>APADNAADARPVDVSVSIFINKIYGVNTLEQTYKVDGYIVAQWTGKPRKTPGDKPLIVENTQIERWINNGLWVPALEFINVVGSPDTGNKRLMLFPDGRVIYNARFLGSFSNDMDFRLFPFDRQQFVLELEPFSYNNQQLRFSDIQVYTENIDNEEIDEWWIRGKASTHISDIRYDHLSSVQPNQNEFSRITVRIDAVRKIGYFVIQTYLPCIMTVILSQVSFWLNRESVPARTVFGVTTVLTMTTLSISARNSLPKVAYATAMDWFIAVCYAFVFSALIEFATVNYFTKRGVESVSKIDRLSRIAFPLLFGIFNLVYWATYLN[10x]

Type A γ-aminobutyric acid receptors (GABAARs) control neuronal excitability and are the primary inhibitory pentameric ligand-gated ion channels (pLGICs) in the central nervous system. GABAAR-mediated inhibition of neuronal excitability results from membrane hyperpolarization due to Cl− flux upon GABAAR activation, which can be triggered by binding of the neurotransmitter GABA to the orthosteric site in the extracellular domain (ECD) or allosteric binding of endogenous neuroactive steroids. Here, we report crystal structures of an α1GABAAR chimera in the apo state and in an alphaxalone-bound desensitized state. The final residue R199 in the ECD of ELIC was fused with the first residue K222 in the TMD of human α1GABAAR.

Alphaxalone (5α-pregnan-3α-ol-11,20 dione) is a potent neurosteroid anesthetic. The structure of the α1GABAAR chimera co-crystallized with alphaxalone shows that alphaxalone binds to five equivalent inter-subunit sites close to the intracellular end of the α1GABAAR TMD. Residues within 4-Å of alphaxalone are from TM3 of the principal subunit (A305, T306, Y309, and F310) and from TM1 (Q242, V243, W246) and TM4 (P401) of the neighboring complementary subunit. The aromatic ring of the conserved residue W246 is parallel to the C ring of alphaxalone, establishing a ring stacking interaction that potentially stabilizes the binding. The pore profile of the α1GABAAR chimera desensitized by alphaxalone is similar to the pore profile of the apo chimera, except that the most constricted pore is located at P253 (−2′) in the desensitized structure. Relative to the aligned structure of the apo ELIC-α1GABAAR, the alphaxalone-bound structure shows 1.3° inward and 0.18° outward radial tilt from the pore axes in the ECD and TMD, respectively. The alphaxalone-bound structure shows a small counterclockwise twist (0.80°) of the ECD and a clockwise twist (1.37°) of the TMD around the pore axis. Alphaxalone binding to the bottom of the TMD introduces structural changes, including the orientation of W246 in the TM1, presumably to optimize its interaction with alphaxalone. The change passes to the TM1–TM2 linker and further to the TM2, particularly at P253 (−2′) and V257 (2′), resulting in a backbone RMSD of 0.95 Å for the residues covering from W246 in TM1 to V257 (2′) in TM2. The structural changes further propagate up to the ECD–TMD interface and other ECD regions, as evidenced by the observed RMSDs: 0.66 Å for the TM2–TM3 loop (P278-T284), 0.61 Å for the pre-TM1 (R199-I223), 0.58 Å for the β1–β2 linker (V26-E30), 0.63 Å for the Cys-loop (N112-F126), 1.01 Å for loop A (N80-S84), and 0.84 Å for loop C (D172-N186).> EVYDVTIIGGGPIGLFTAFYCGMRELKTKVIEFLPKLGGKVSLFFPEKIIRDIGGIPGIAGKQLIEQLKEQAATFDPDIVLNQRVTGFERLDDGTIVLTGSEGKKHYTRTVILACGMGTLEVNEFDSEDAARYAGKNLHYGVEKLDAFKGKRVVISGGGDTAVDWANELEPIAASVTVVHRREEFGGMESSV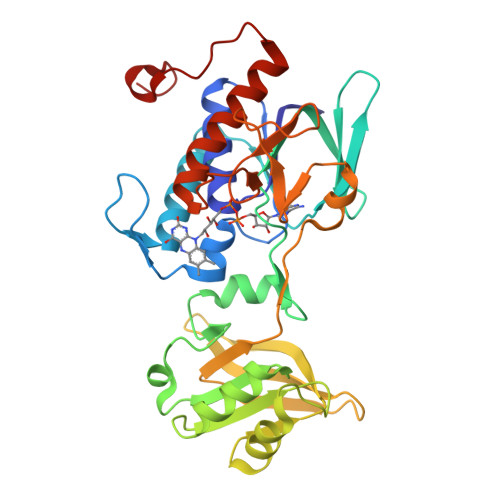TKMKQSSVRVLTPYRLEQLNGDEEGIKSVTVCHTESGQRKDIEIDELIINHGFKIDLGPMMEWGLEIEEGRVKADRHMRTNLPGVFVAGDAAFYESKLRLIAGGFTEGPTAVNSAKAYLDPKAENMAMYSTHHKKLV> RSLIANNTVN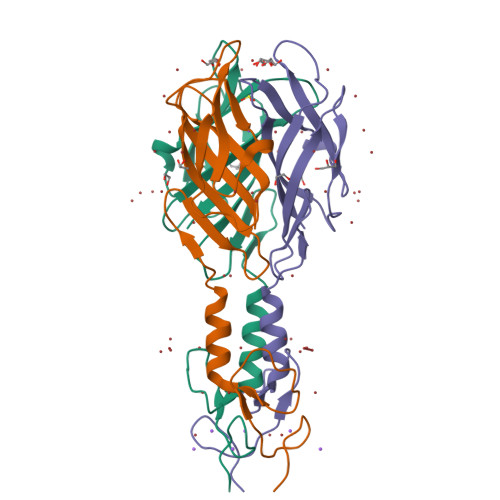PNNGLGGAWEVYSGQGSIPTATSTTAGITKVLNVLNSNDVGSALSAAQGKVLNDKFNFQNSKNQSGYVRLGDSGLIIQWGVFTSTKTQSNLIFPLAFPNALLSITGNLNSNTPDVIGIDFDLSTATKTSIKTGAAQVGASWLSGKKISWIAIGY> APLADYKDDDDKLAGATWTTRGFVFTRHSQTTAIPSCPEGTVPLYSGFSFLFVQGNQRAHGQDLGTLGSCLQRFTTMPFLFCNVNDVCNFASRNDYSYWLSTPALMPMNMAPITGRALEPYISRCTVCEGPAIAIAVHSQTTDIPPCPHGWISLWKGFSFIMFTSAGSEGTGQALASPGSCLEEFRASPFLECHGRGTCNYYSNSYSFWLASLNPERMFRKPIPSTVKAGELEKIISRCQVCMGTGFLLVLHSQTDQEPTCPLGMPRLWTGYSLLYLEGQEKAHNQDLGLAGSCLPVFSTLPFAYCNIHQVCHYAQRNDRSYWLASAAPLPMMPLSEEAIRPYVSRCAVCEAPAQAVAVHSQDQSIPPCPQTWRSLWIGYSFLMHTGAGDQGGGQALMSPGSCLEDFRAAPFLECQGRQGTCHFFANKYSFWLTTVKADLQFSSAPAPDTLKESQAQRQKISRCQVCVAPGFLITRHSQTTDAPQCPQGTLQVYEGFSLLYVQGNKRAHGQDLGTAGSCLRRFSTMPFMFCNIN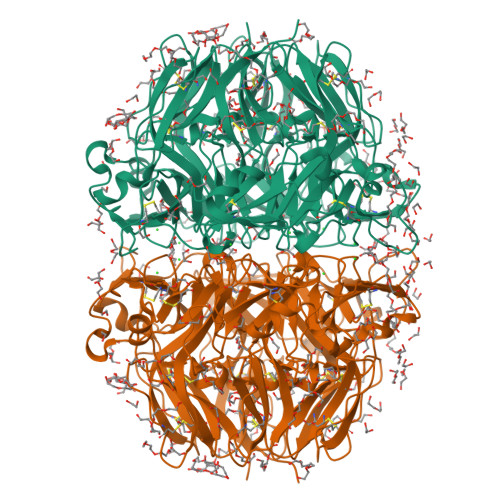NVCNFASRNDYSYWLSTPEPMPMSMQPLKGQSIQPFISRCAVCEAPAVVIAVHSQTIQIPHCPQGWDSLWIGYSFMMHTSAGAEGSGQALASPGSCLEEFRSAPFIECHGRGTCNYYANSYSFWLATVDVSDMFSKPQSETLKAGDLRTRISRCQVCMKRT>[2x]MRKNRGFSVSSKAVMMCCLAFLLIPASFAFAAPNKPFPQHTTYTSGSIKPNHVTQSAMDNSVKAKWDSWKSAYLKTAGTGKYYVKYQSNGDTVSEAHGYGMLATVLMAGYDSNAQTYFDGLYQYYKAHPSSNNSKL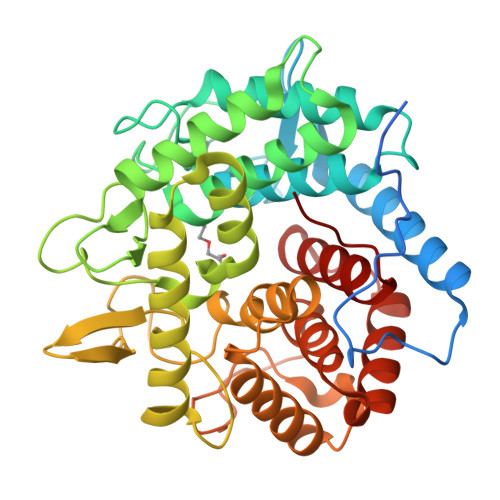MAWKQNSSFQNIEGDDSATDGDMDIAYSLLLADKQWGSSGSINYLQAGKDIINAIMQSDVNQSQWTLRLGDWATDNTFKNATRPSDFMLNHLKAFQAATGDARWANVIDKTYTIINSLYNGYSSSTGLLPDFVVLSGSTYKPASADFLEGANDGSYDYNSCRTPWRITTDYLMTGDSRALNQLNQMNSWISAKVSGNPSNVKDGYKLNGTVTGSGGSGAFYAPFGVSAMTSSVNQNWLNSVWTKTAGSSNEGYYEDSIKLFSMIVMSGNWWTY>[8x]ENRPVALIT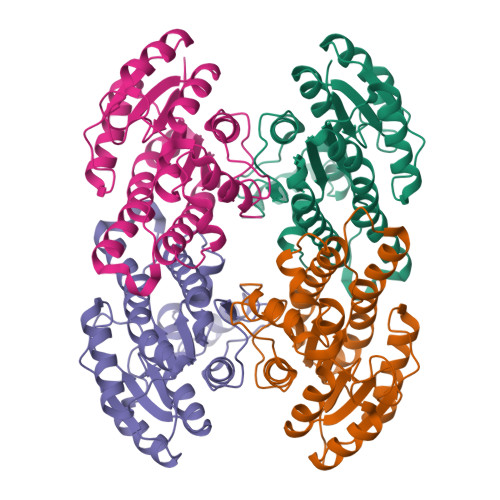MATGYVGPALARTMADRGFDLVLHGTAGDGTMVGVEESFDSQIADLAKRGADVLTISDVDLTTRTGNQSMIERVLERFGRLDSACLVTGLIVTGKFLDMTDDQWAKVKAGNLDMVFHGLQAVLPPMVAAGAGQCVVFTSATGGRPDPMVSIYGGTRAGANGIVRAVGLEHARHGVQVNAIGTNYMDFPGFLKASRADGDPERRAMIEAQVPLRRLGTMDELSSVTAGLLDGSNRFQTGQFFDFSGGWGA4-((1-(2-(2-(2-(2-hydroxyethoxy)ethoxy)ethoxy)ethyl)-1H-1,2,3-triazol-4-yl)methoxy)benzyl-a-L-thiofucoside 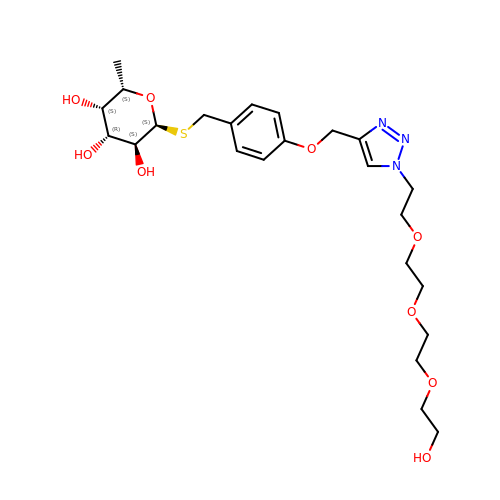| C24 H37 N3 O9 S | YKPIHJOKBVPCNG-BQEPTVRSSA-N>[2x]EIGTGFPFDPHYVEVLGSRMHYVDVGPRDGTPVLFLHGNPTSSYLWRNIIPHVAPSHRCIAPDLIGMGKSDKPDLDYRFDDHVRYLDAFIEALGLEEVVLVIHDWGSALGFHWAKRNPERVKGIAFMEFIRPIPTWDEWPEFARELFQAFRTPDVGRELIIDQNAFIEGILPKFVVRPLTEVEMDHYREPFLKPVWREPLWRFPNELPI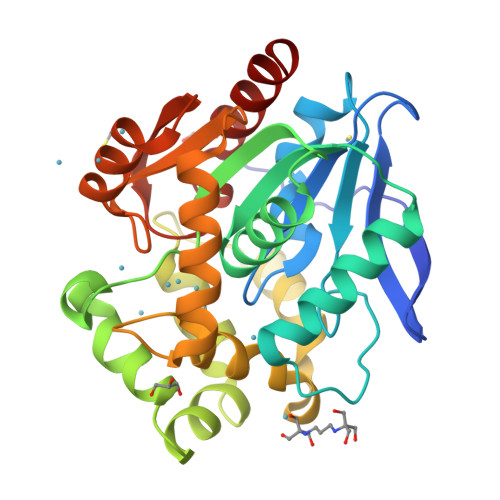AGEPANIWALVEAYMNWLHQSPVPKLLFWGTPGVLIPPAEAARLAESLPNLKTVFIGPGLHYLQEDNPDLIGSEIARWLPAL>[3x]MATAAEIAALPRQKVELVDPPFVHAHSQVAEGGPKVVEFTMVIEEKKIVIDDAGTEVHAMAFNGTVPGPLMVVHQDDYLELTLINPETNTLMHNIDFHAATGALGGGGLTEINPGEKTILRFKATKPGVFVYHCAPPGMVPWHVVSGMNGAIMVLPREGLHDGKGKALTYDKIYYVGEQDFYVPRDENGKYKKYEAPGDAYEDTVKVMRTLT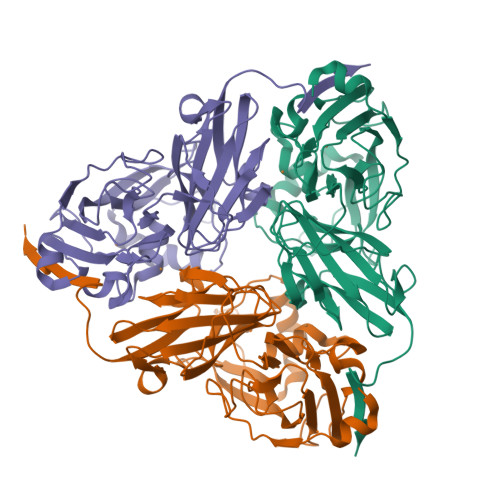PTHVVFNGAVGALTGDKAMTAAVGEKVLIVHSQANRDTRPHLIGGHGDYVWATGKFNTPPDVDQETWFIPGGAAGAAFYTFQQPGIYAYVNHNLIEAFELGAAAHFKVTGEWNDDLMTSVLAPSGTLVPR> GPTAAAAMGRGVPHIVMVDAYKRYK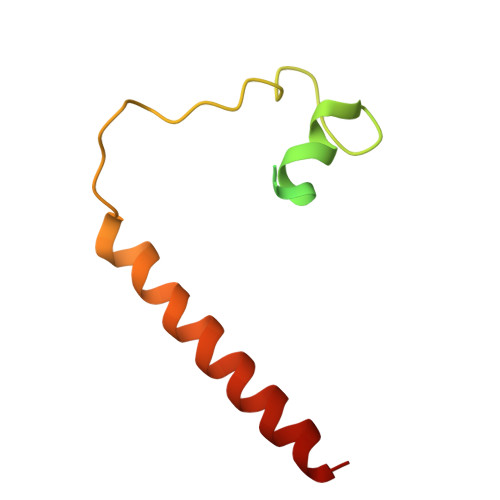GGGSGGSGGGMVHVLERALLEQQSSACGLPGSSTETRPSHPCPEDPDVSRLRLLLVVLCVLFGLLCLLLI> SFFFLSFHISNLQFNSSLEDPSTDYYQELQRDISEMFLQIYKQGGFLGLSN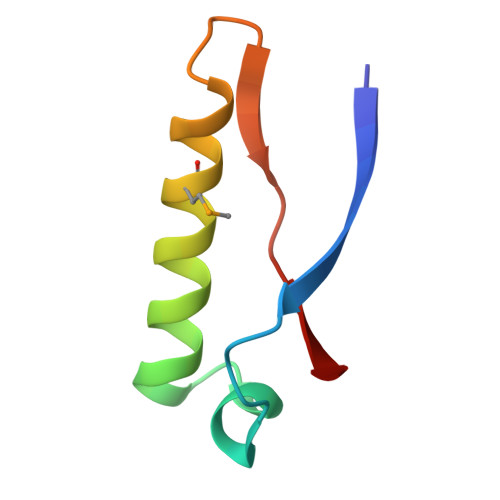IKFRPG>[2x]AGPTAVPLGTAGNY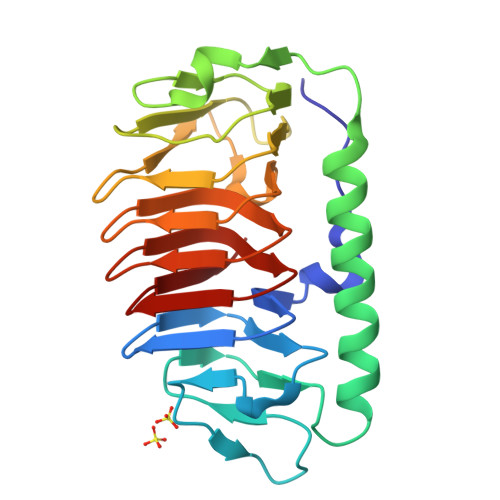AILASTAVSTVPQSAITGAVGISPAAGTFLTGFSLTMSGTGTFSTSTQVTGQLTAADYGTPTPSILTTAIGDMGTAYTNGATRSGPDFLEIYTGALGGTTLLPGLYKWTSSVGASADFTISGTSTDTWIFQIDGTLGLAAGKKITLAGGAQAKNIIWVVAGAVSIEAGAQFEGVILAKTAVTLKTGSSLNGRILAQTSVALQSATVVQK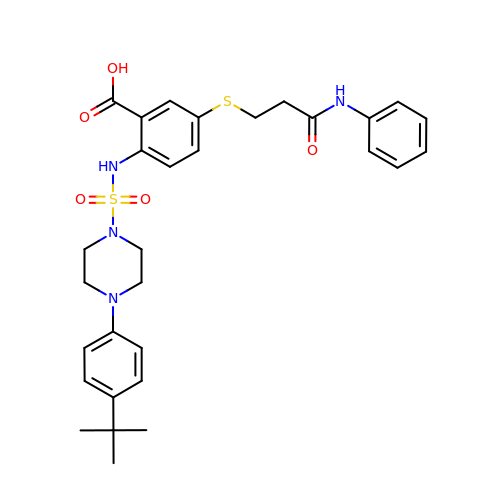2-({[4-(4-tert-butylphenyl)piperazin-1-yl]sulfonyl}amino)-5-{[3-oxo-3-(phenylamino)propyl]sulfanyl}benzoic acid | C30 H36 N4 O5 S2 | STJXGZZMVAELRV-UHFFFAOYSA-N> PAFIVNTNVPRASVPEGFLSELTQQLAQATGKPAQYIAVHVVPDQLMTFSGTSDPCA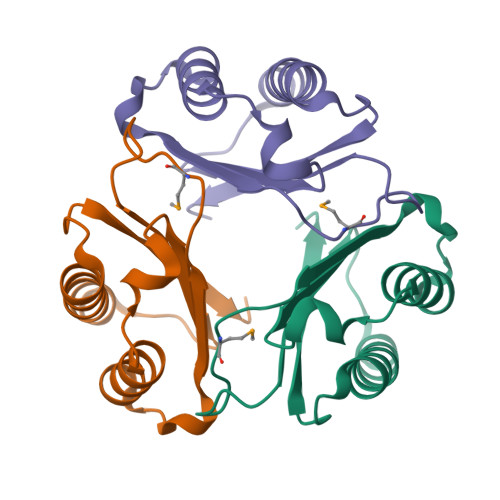LCSLHSIGKIGGAQNRNYSKLLCGLLSDRLHISPDRVYINYYDANAANVGWNGSTFA>[2x]GPLGSPQFMNPAAEAEFNILLATDSYKVTHYKQYPPNTSKVYSYFECREKKTENSKLRKVKYEETVFYGLQYILNKYLKGKVVTKEKIQEAKDVYKEHFQDDVFNEKGWNYILEKYDGHLPIEIKAVPEGFVIPRGNVLFTVENTDPECYWLTNWIETI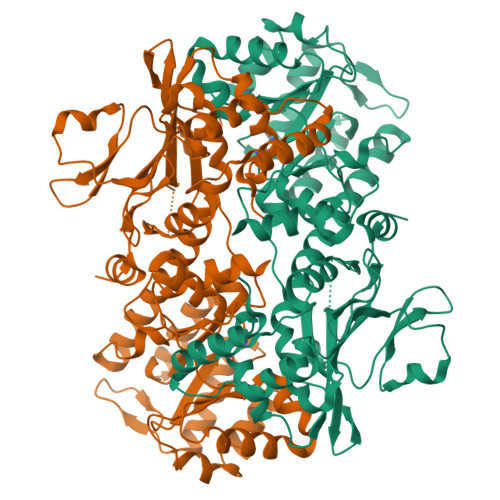LVQSWYPITVATNSREQKKILAKYLLETSGNLDGLEYKLHDFGYRGVSSQETAGIGASAHLVNFKGTDTVAGLALIKKYYGTKDPVPGYSVPAAEHSTITAWGKDHEKDAFEHIVTQFSSVPVSVVSDSYDIYNACEKIWGEDLRHLIVSRSTQAPLIIRPDSGNPLDTVLKVLEILGKKFPVTENSKGYKLLPPYLRVIQGDGVDINTLQEIVEGMKQKMWSIENIAFGSGGGLLQKLTRDLLNCSFKCSYVVTNGLGINVFKDPVADPNKRSKKGRLSLHRTPAGNFVTLEEGKGDLEEYGQDLLHTVFKNGKVTKSYSFDEIRKNAQLNIELEAAHH>[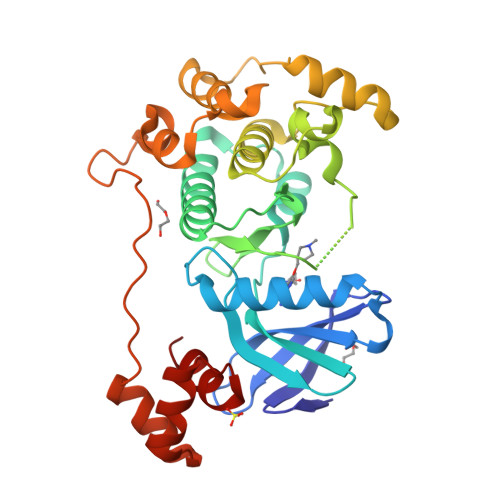2x]QPHIGNYRLLKTLGKGNFAVVKLARHILTGKEVAIKIIDKTQLNSSSLQKIFREVRIMKVLNHPNIIKLFEVIETEKTLYLVTEYAKNGEVFDYLVAHGRMKEKEARAKFRQIVSAVQYCHQKFIVHRDLKAENLLLDADMNIKIADFGFGNEFTFGNKLDTFCGSPPYAAPELFQGKKYDGPEVDVWSLGVILYTLVSGSLPFDGQNLKELRERVLRGKYRIPFYMSTDCENLLKKFLILNPSKRGTLEQIMKDRWMNVGHEDDELKPYVEPLPDYKDPRRTELMVSMGYTREEIQDSLVGQRYNEVMATYLLLGY> GSMELLQGKTFVVMGVANQRSIAWGIARSLHNAGAKLIFTYAGERLERNVRELADTLEGQESLVLPCDVTNDEELTACFETIKQEVGTIHGVAHCIAFANRDDLKGEFVDT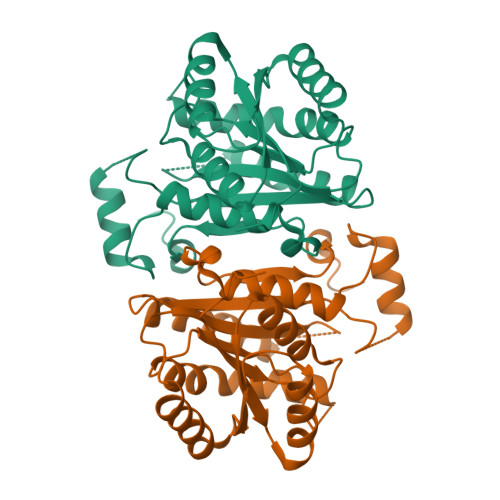SRDGFLLAQNISAFSLTAVAREAKKVMTEGGNILTLTYLGGERVVKNYNVMGVAKASLEASVKYLANDLGQHGIRVNAISAGPIRTLSAKGVGDFNSILREIEERAPLRRTTTQEEVGDTAVFLFSDLARGVTGENIHVDSGYHILGLEHHHHHH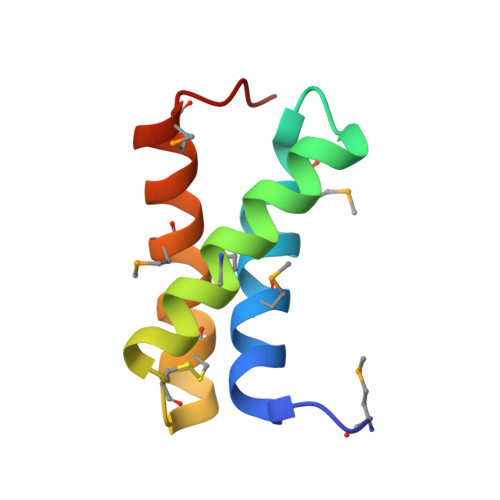> MNVDPHFDKFMESGIRHVYMLFENKSVESSEQFYSFMRTTYKNDPCSSDFECIERGAEMAQSYARIMNIKLETE> MNDAAEVALYERLLQLRVLPGASDVHDVRFVFGDDSRCWIEVAMHGDHVIGNSHPALDPKSRATLEHVLTVQGDLAAFLVVARDMLLASL;> GSHMEANENILKLKLYRSLGVILDLEN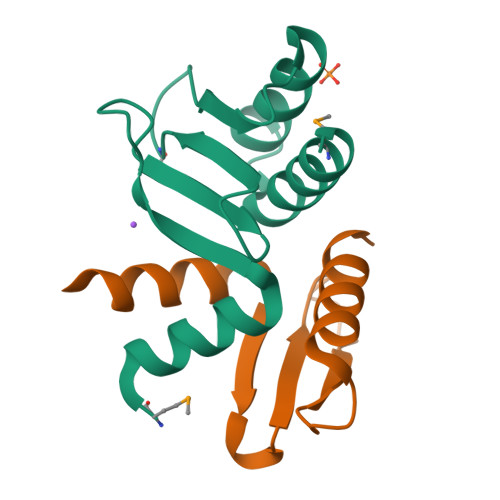DQVLINRKNDGNIDILPLDNNLSDFYKTKYIWERLGK> MVGGGVIRQLLRRKLHSQSVATPVLSWLSSKKANEDAGSAGLRAFALMGAGITGLLSFSTVASADEAEHGLECPNYPWPHEGILSSYDHASIRRGHQVYQQVCASCHSMSLISYRDLV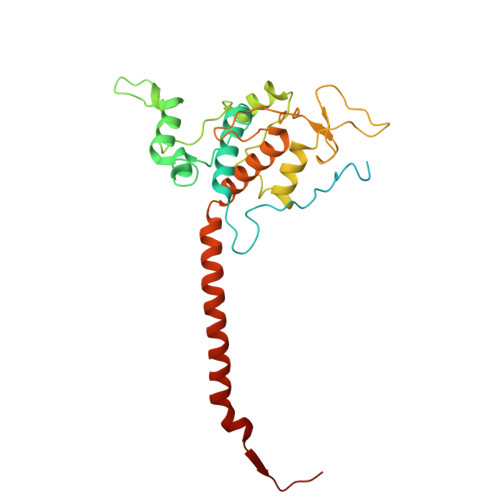GVAYTEEEAKAMAAEIEVVDGPNDEGEMFTRPGKLSDRLPEPYSNESAARFANGGAYPPDLSLVTKARHNGQNYVFALLTGYRDPPAGISIREGLHYNPYFPGGAIAMPKMLNDEAVEYEDGTPATEAQMGKDVVSFLSWAAEPEMEERKLMGFKWIFLLSLALLQAAYYRRLKWSVLKSRKLVLDVVN>[2x]GPVSVANHLGEDAGHLALRRDVYSGLQKTPKSLPPKWFYDTVGSELFDQITRLPEYYPTRAEAEILRARSAEVASACRADTLVELGSGTSEKTRMLLDALRHRGSLRRFVPFDVDASVLSATATAIQREYSGVEINAVCGDFEEHLTEIPRGGRRLFVFLGSTIGNLTPGPRAQFLTALAGVMRPGDSLLLGTDLVKDAARLVRAYDDPGGVTAQFNRNVLAVINRELEADFDVDAFQHVARWNSAEERIEMWLRADGRQRVRVGALDLTVDFDAGEEMLTEVSCKFRPQAVGAELAAAGLHRIRWWTDEAGDFGLSLAAK

EgtD, an S-adenosylmethionine-dependent methyltransferase (AdoMet), catalyzes the trimethylation of L-Histidine to initiate EGT biosynthesis and this reaction has been shown to be essential for EGT production in mycobacteria and for long-term infection of murine macrophages by M. tb. Synthesis of EGT by Mycobacterium tuberculosis (M. tb) is critical for maintaining bioenergetic homeostasis and protecting the bacterium from alkylating agents, oxidative stress, and anti-tubercular drugs. Multiple X-ray crystal structures of Mycolicibacterium smegmatis EgtD show that EgtD possesses a Histidine binding domain and a Rossmann-fold domain, which affords ordered substrate binding of L-Histidine and AdoMet, respectively. In this work, library screening and structure-guided strategies identified multiple classes of M. tb EgtD inhibitors that bind in various regions of the enzyme active site.

The obtained crystals were subjected to X-ray diffraction experiments and X-ray crystal structures were obtained for M. tb EgtD with HD2, HD3, and HD6. HD2 forms primarily polar interactions with the histidine binding site residues of EgtD. Specifically, HD2 forms a hydrogen-bonded interaction between an ordered water molecule, positioned by the Thr213 side chain and the backbone carbonyl of Ala205, and the basic nitrogen atom of the imidazole moiety. As with L-Histidine in published EgtD structures, the carboxylic group in HD2 forms hydrogen-bonded interactions with Tyr206, Ser284, and Tyr56. This compound is commercially available as a racemic mixture of L- and D- HD2 enantiomers. Based on the interactions observed in the EgtD complex with L-Histidine, it is reasonable to expect the L-enantiomer to be the dominant ligand. In this case, the 2.7 Å resolution of the EgtD-HD2 complex X-ray crystal structure is not sufficient to unambiguously define the stereochemistry of the bound inhibitor. The pyrrole moiety of HD2 forms a 3.6 Å van der Waals interaction with the α-carbon of Thr163 and a 3.3 Å van der Waals interaction with the side chain of Asn166. First, HD2, HD3, and HD6 most closely resemble a Histidine amino acid as they all possess α-amino and α-carboxyl moieties, but the α-amino group is elaborated with a variety of chemical linkages. As expected, these binding modes closely resemble that of L-Histidine with the minor exception of the α-carboxylate moiety of HD3.>HLDIPEDYQERLQAEPFTDCVPMLRLEFTGQSVDAPLLSETARRFN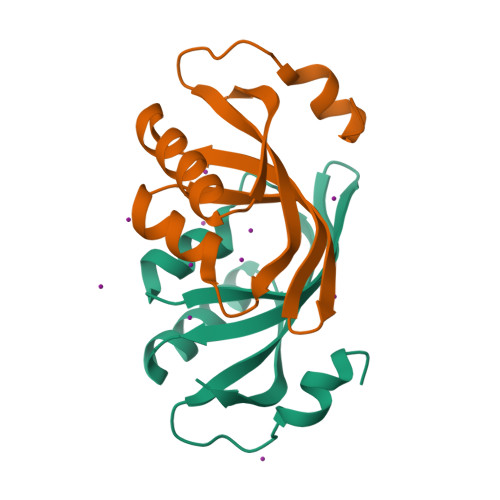VNNNIISAQMDYAGGVKFGIMLTEMHGTQQDTQAAIAWLQEHHVKVEVLGYVLEHHHHHH[2x]> MDFITDMSKNQRLELQNRLAQYETSLMVMSHNGDVPVITGFNVMRVTTMLDALKVELPAVAVLGDDAQDLAYVFGARPLAVGVNIIRVVDVPGQQPSALVDAELGALHEVSMVRVLND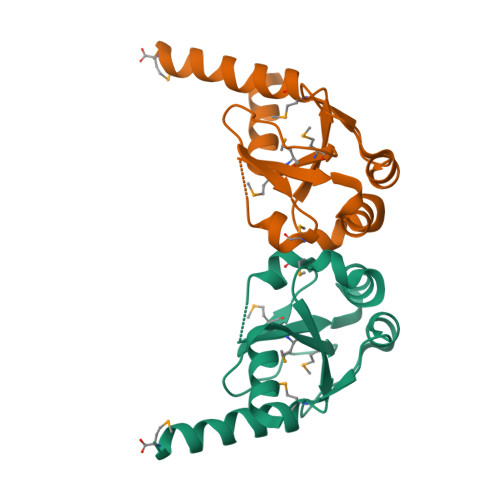IADEQLVKANM> MAATAAEAVASGSGEPREEAGALGPAWDESQLRSYSFPTRPIPRLSQSDPRAEELIENEEPVVLTDTNLVYPALKWDLEYLQENIGNGDFSVYSASTHKFLYYDEKKMANFQNFKPRSNREEMKFHEFVEKLQDIQQRGGEERLYLQQTLNDTVGRKIVMDFLGFNWNWINKQQGKRGWGQLTSNLLLIGMEGNVTPAHYDEQQNFFAQIKGYKRCILFPPDQFECLYPYPVHHPCDRQSQVDFDNPDYERFPNFQNVVGYETVVGPGDVLYIPMYWWHHIESLLNGGITITVNFWYKGAPTPKRIEYPLKAHQKVAIMRNIEKMLGEALGNPQEVGPLLNTMIKG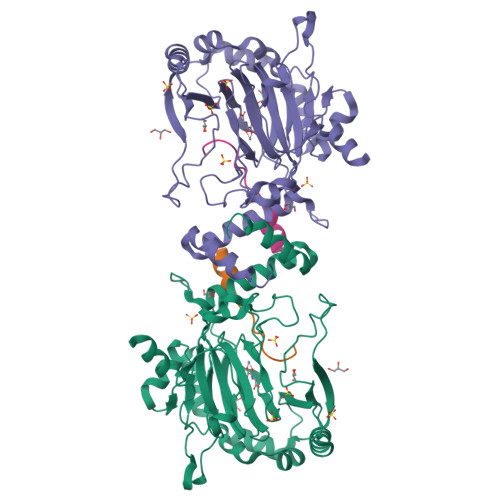RYN;> EVVKLLLEHGADVLAQD>[2x]QNRTVKGTVISSEDNEPLIGANVVVVGNTTIGAATDLDGNFTLSVPANAKMLRVSYSGMTTKEVAIANVMKIVLDPDSKVLEQVVVLGYGTGQKLSTVSGSVAKVSSEKLAEKPVANIMDALQGQVAGMQVMTTSGDPTAVASVEIHGTGSLGASSAPLYIVDGMQTSLDVVATMNPNDFESMSVLKDASATSIYGARAANGVVFIQTKKGKMSERGRITFNASYGISQILNTKPLDNMMTGDELLDFQVKAGFWGNNQTVQKVKDMILAGAEDLYGNYDSLKDEYGKTLFPVDFNHDADWLKALFKTAPTSQGDISFSGGSQGTSYYASIGYFDQEGMAREPANFKRYSGRLNFESRINEWLKVGANLSGAIANRRSADYFGKYYMGSGTFGVLTMPRYYNPFDVNGDLADVYYMYGATRPSMTEPYFAKMRPFSSESHQANVNGFAQITPIKGLTLKAQAGVDITNTRTSSKRMPNNPYDSTPLGERRERAYRDVSKSFTNTAEYKFSIDEKHDLTALMGHEYIEYEGDVIGASSKGFESDKLMLLSQGKTGNSLSLPEHRVAEYAYLSFFSRFNYGFDKWMYIDFSVRNDQSSRFGSNNRSAWFYSVGGMFDIYNKFIQESNWLSDLRLKMSYGTTGNSEIGNYNHQALVTVNNYTEDAMGLSISTAGNPDLSWEKQSQFNFGLAAGAFNNRLSAEVDFYVRTTNDMLIDVPMPYISGFFSQYQNVGSMKNTGVDLSLKGTIYQNKDWNVYASANFNYNRQEITKLFFGLNKYMLPNTGT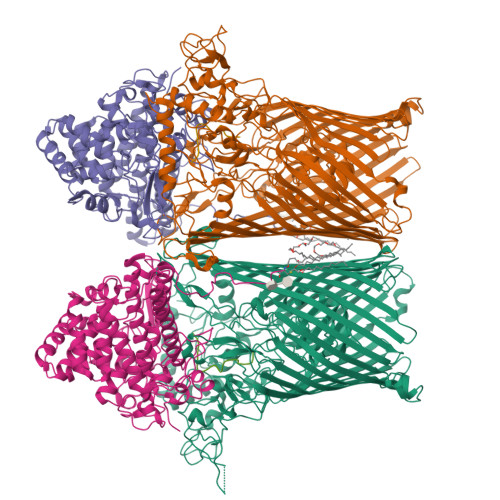IWEIGYPNSFYMAEYAGIDKKTGKQLWYVPGQVDADGNKVTTSQYSADLETRIDKSVTPPITGGFSLGASWKGLSLDADFAYIVGKWMINNDRYFTENGGGLMQLNKDKMLLNAWTEDNKETDVPKLGQSPQFDTHLLENASFLRLKNLKLTYVLPNSLFAGQNVIGGARVYLMARNLLTVTKYKGFDPEAGGNVGKNQYPNSKQYVAGIQLSF;>CELDRDPEGKDFQQPYTSFVQTKQNRDGLYALLRNTENPRMHFYQELQSDMYCTTITDGNSLAPFVNWDLGILNDHGRADEDEVSGIAGYYFVYNRLNQQANAFVNNTEAALQNQVYKNSTEIANAKSFLAEGKVLQALAIWRLMDRFSFHESVTEVNSGAKDLGVILLKEYNPGYIGPRATKAQCYDYILSRLSEAIEVLPENRESVLYVSRDYAYALRARIYLALGEYGKAAADAKMVVDKYPLIGAADASEFENIYRSDANNPEIIFRGFASATLGSFTATTLNGAAPAGKDIKYNPSAVPFQWVVDLYENEDFRKSVYIAKVVKKDKGYLVNKFLEDKAYRDVQDKPNLKVGARYFSVAEVYLILVESALQTGDTPTAEKYLKALSKARGAEVSVVNMEALQAERTRELIGEGSRLRDMVRWSIPNNHDAFETQPGLEGFANTTPLKAQAPVGFYAYTWEFPQRDRQTNPQLIKNWPIHHHHHH[2x];> ASTTGANSQRGSG;> ASTTGANSQR> MDSFPLLAALFFIAATITFLSFRRRRNLPPGPFPYPIVGNMLQLGANPHQVFAKLSKRYGPLMSIHLGSLYTVIVSSPEMAKEILHRHGQVFSGRTIAQAVHACDHDKISMGFLPVASEWRDMRKICKEQMFSNQSMEASQGLRRQKLQQLLDHVQKCSDSGRAVDIREAAFITTLNLMSATLFSSQATEFDSKATMEFKEIIEGVATIVGVPNFADYFPILRPFDPQGVKRRADVFFGKLLAKIEGYLNERLESKRANPNAPKKDDFLEIVVDIIQANEFKLKTHHFTHLMLDLFVGGSDTNTTSIEWAMSELVMNPDKMARLKAELKSVAGDEKIVDESAMPKLPYLQAVIKEVMRIHPPGPLLLPRKAESDQEVNGYLIPKGTQILINAYAIGRDPSIWTDPETFDPERFLDNKIDFKGQDYELLPFGSGRRVCPGMPLATRILHMATAT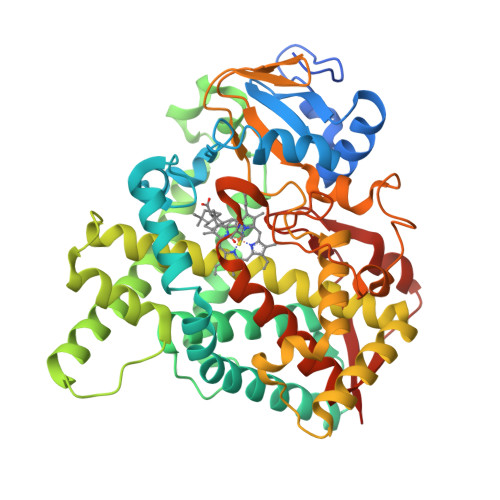LVHNFDWKLEDDSTAAADHAGELFGVAVRRAVPLRIIPIVKS> M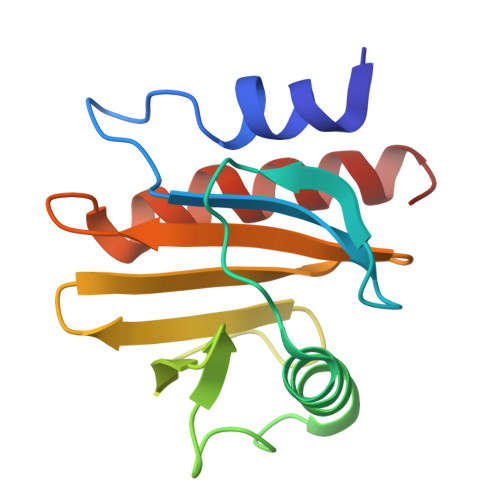SWQSYVDDHLMCEVEGNHLTHAAIFGQDGSVWAQSSAFPQLKPAEIAGINKDFEEAGHLAPTGLFLGGEKYMVVQGEAGAVIRGKKGPGGVTIKKTTQALVFGIYDEPMTGGQCNLVVERLGDYLIESGL The similarity of eukaryotic actin to crenactin, a filament-forming protein from the crenarchaeon Pyrobaculum calidifontis supports the theory of a common origin of Crenarchaea and Eukaryotes. Attempts to trace back the origins of today's eukaryotic F-actin filaments led to the discovery of crenactin found in certain organisms of the order Thermoproteales within the phylum Crenarchaeota (Crenarchaea, part of the 'TACK' superphylum). Hence, it has been proposed that crenactin filaments share a common ancestor with F-actin. In Pyrobaculum calidifontis, crenactin is encoded within the arcade cluster of genes, together with four arcadins, and has been proposed to be part of a cell-shape maintenance system.

Arcadin-2 depolymerises crenactin filaments by binding its C-terminus into crenactin's hydrophobic groove, a mode of action related to eukaryotic actin modulators, widening the potential evolutionary links. Addition of a C-terminally truncated version of arcadin-2 had no effect, suggesting that the conserved C-terminal α-helix of arcadin-2 was responsible for the depolymerisation of crenactin filaments. Indeed, the peptide triggered depolymerisation of the filaments at a similar rate as full-length arcadin-2. This effect was confirmed by analytical ultra centrifugation, showing that crenactin becomes monomeric upon addition of the C-terminal arcadin-2 peptide. Co-expression and subsequent purification of crenactin and arcadin-2 resulted in a tight 1:1 complex. The dissociation constant of this complex was very low with a Kd of 31 ± 4 nM (n = 4), as measured by SPR (Surface Plasmon Resonance). To gain a better understanding of this interaction, how it triggers depolymerisation and how this might be related to F-actin depolymerisation, we solved the crystal structure of crenactin in complex with arcadin-2 C-terminal peptide. The structure was solved to 1.6 Å by X-ray crystallography providing detailed insights into crenactin, binding to ATP and, more importantly, showing how arcadin-2 induced depolymerisation of the filaments. The arcadin-2 peptide was located in the hydrophobic groove on crenactin, a cavity formed between subdomains IA and IIA. In the filament, this hydrophobic groove is occupied by the D-loop of the following subunit in a strand, forming one half of the longitudinal contact. The nanomolar interaction between arcadin-2 peptide and the hydrophobic pocket is likely due to a tryptophan and other hydrophobic residues, making strong contacts as shown in Figure 3—figure supplement 2E.

> MGVISDAYRLKYTFGVDFGTSYVKYGPITLNEPKMVQTRGLFLRDLPESVKMRIPPDVLARGLVVGDEEVRKYLSSVRDVQRNLKYPLKDGVARRDDEEAWRVLKELARYTLAQFPVSDPEFAGWLVAVALSALAPDYMYKAIFDIYDELASEFKIYAVTILPQPLAVAIAENAVNCVIVEGGHGNIQVAPISFALIREGLVALNRGGAEANAITREILKDIGYSDIAREEYAVEVVKRAVGLVPRRLKEAIRAAKSDPDRFVTKVRLSPVVEVEIPREYAWTRFLIGEIVFDPNHEEIKSYIEQSRLRIENAVIGDVTLYGEMDVASAIITSLRNVSVEIQERVASQIILSGGAFSWRVPPGMEDVAADSVTRVKIALEEKSPALASKVEVRLVSEPQYSVWRGAVIYGYALPLSLEWSDTTREGWRFPRR;> GGIGENEWVKILRSKR>ASRYLTDMTLEEMSRDWFMLMPKQKVAGSLCIKMDQAIMDKTIILKANFSVIFDRLETLILLRAFTEEG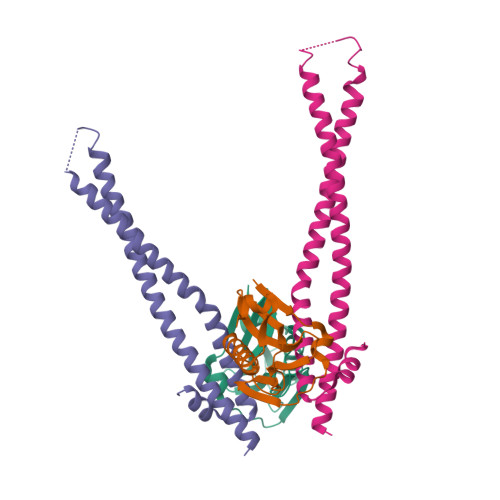AIVGEISPLPSLPGHTGEDVKNAIGVLIGGLEANDNTVRVTETIQRFAWRNSDEDGR[2x];>GSKEDSVEAVGAQLKVYHQQYQDKSREYDQLYEEYTRTSQELQMKRTAIEAFNETIKIFEEQGQTQEKCSKEYLERFRREGNEKEMQRILLNSERLKSRIAEIHESRTKLEQQLRAQASDNREIDKRMNSLKPDLMQLRKIRDQYLVWLTQKGARQKKINEWLGI[2x]>MGVEDEPLLRENPRRFVIFPIEYHDIWQMYKKAEASFWTAEQVDLSKDIQHWESLKPEERYFISHVLAFFAASDGIVNENLVERFSQEVQITEARCFYGFQIAMENIHSEMYSLLIDTYIKDPKEREFLFNAIETMPCVKKKADWALRWIGDKEATYGERVVAFAAVEGIFFSGSFASIFWLKKRGLMPGLTFSNELISRDEGLHCDFACLMFKHLVHKPSEERVREIIINAVRIEQEFLTEALPVKLIGMNCTLMKQYIEFVADRLMLEL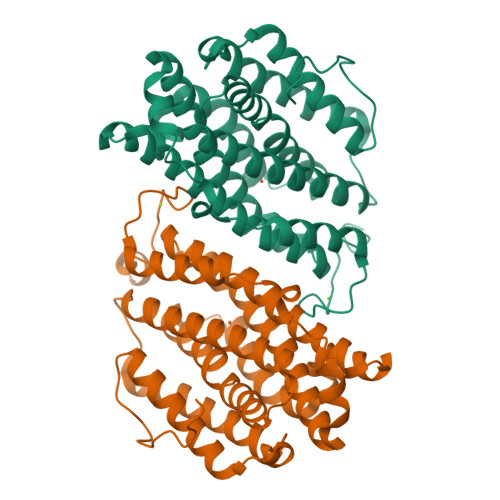GFSKVFRVENPFDFM[2x]>MSKPSIVILGAGYGGIVAALGLQKRLNYNEADITLVNKNDYHYITTELHQPAAGTMHHDQARVGIKELIDEKKIKFVKDTVVAIDREQQKVTLQNGELHYDYLVVGLGSEPETFGIEGLREHAFSINSINSVRIIRQHIEYQFAKFAAEPERTDYLTIVVGGAGFTGIEFVGELADRMPELCAEYDVDPKLVRIINVEAAPTVLPGFDPALVNYAMDVLGGKGVEFKIGTPIKRCTPEGVVIEVDGEEEEIKAATVVWTGGVRGNSIVEKSGFETMRGRIKVDPYLRAPGHENIFIVGDCALIINEENNRPYPPTAQIAIQHGENVAANLAALIRGGSMTPFKPHIRGTVASLGRNDAIGIVGGRKVYGHAASWLKKLEDMRYLYLIGGLSLVLKK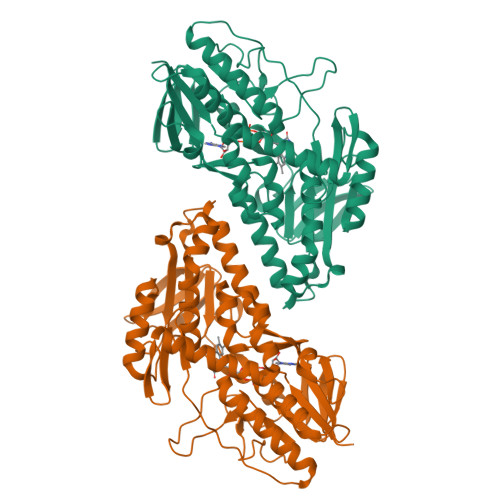GRFHHHHHH[4x]>SSNDNIELVDFQNIMFYGDAEVGDNQQPFTFILDTGSANLWVPSVKCTTAGCLTKHLYDSSKSRTYEKDGTKVEMNYVSGTVSGFFSKDLVTVGNLSLPYKFIEVIDTNGFEPTYTASTFDGILGL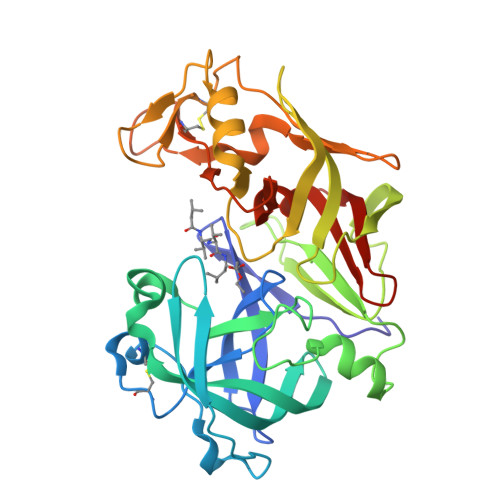GWKDLSIGSVDPIVVELKNQNKIENALFTFYLPVHDKHTGFLTIGGIEERFYEGPLTYEKLNHDLYWQITLDAHVGNIMLEKANCIVDSGTSAITVPTDFLNKMLQNLDVIKVPFLPFYVTLCNNSKLPTFEFTSENGKYTLEPEYYLQHIEDVGPGLCMLNIIGLDFPVPTFILGDPFMRKYFTVFDYDNHSVGIALAKKNL[2x]Poliovirus (PV) belongs to the Enterovirus genus of the Picornaviridae family. The PV genome, approximately 7.5 kb in length, is a single-stranded, positive-sense RNA enclosed within a capsid protein shell. The P1 is further cleaved by a viral protease to produce the capsid subunit proteins VP0, VP1, and VP3. In this study, we investigate the production, antigenicity, thermostability, immunogenicity, and structures of VLPs derived from PV serotype 2 (PV2) wildtype strain and thermally stabilized mutant (wtVLP and sVLP, respectively).

The structural comparison showed that the wtVLP is highly similar to the PV1 135S-like particles, and the sVLP structure aligns well with the native PV2 model. These data indicate that the PV2 sVLP adopts a native conformation similar to that of the corresponding mature virion, whereas the PV2 wtVLP is in a non-native expanded state. However, the wtVLP appears to be in an expanded state compared to the sVLP, as evidenced by the radius of the wtVLP being 170 Å and that of the sVLP being 163 Å. Structural comparison revealed that the two-fold axis channel, formed by VP2 and VP3, is markedly opened in the wtVLP, whereas it is closed in the sVLP. Noteworthy, a lipid “pocket factor” modeled as sphingosine was observed within the VP1 “pocket” of the sVLP, while the “pocket” in the wtVLP was empty. In comparison to the PV2 wtVLP, the sVLP contains five amino acid alterations, including VP1 T41I, VP1 F134L, VP1 Y159F, VP3 L85F, and VP3 Q178L. According to our structural analysis, VP1 F134L and Y159F are situated in the VP1 pocket, VP3 Q178L is located at the protomer interface and in proximity to the quasi-three-fold, L85F is present on the VP3 β-sheet, and VP1 T41I, which remains unresolved, is at the pentamer interface within the capsid. In the sVLP, the Q178L mutation transforms the residue from a hydrophilic to a hydrophobic amino acid, thereby enhancing the hydrophobic interaction between protomers. In addition, the residues F134L and Y159F enlarge the “pocket” to accommodate a lipidic pocket factor, which is known to stabilize the particle. While VP4 and the N-terminal (residues 1–68) of VP1 are unresolved in both VLPs, the sVLP, unlike the wtVLP, has ordered structures in the C-terminal of VP1, residues 213–231 in the VP1 GH loop, residues 134–149 and 160–173 in the VP2 EF loop, and the VP3 GH loop. Interestingly, the doorloop 232–236 in our PV2 sVLP was found to be in the “down” conformation whereas it adopts the “up” conformation in the PV2 native virion model.

> GLGDLIEGVVEGVTRNALTPLTPANNLPDTQSSGPAHSKEIPALTAVETGATNPLVPSDTVQTRHVIQKRTRSESTVESFFARGACVAIIEVDNDAPTKRASKLFSVWKITYKDTVQLRRKLEFFTYSRFDMELTFVVTSNYTDANNGHALNQVYQIMFIPPGAPIPGKWNDYTWQTSSNPSVFYTYGAPPARISVPYVGIANAYSHFYDGFAKVPLAGQASTEGDSLYGAASLNDFGSLAVRVVNDHNPTKLTSKIRVYMKPKHVRVWCPRPPRAVPYYGPGVDYKDGLAPLPEKGLTTY;> SPNIEACGYSDRVMQLTLGNSTITTQEAANSVVAYGRWPEYIKDSEANPVDQPTEPDVAACRFYTLDTVTWRKESRGWWWKLPDALKDMGLFGQNMFYHYLGRAGYTVHVQCNASKFHQGALGVFAVPEMCLAGDSTTHMFTKYENANPGEKGGEFKGSFTLDTNATNPARNFCPVDYLFGSGVLAGNAFVYPHQIINLRTNNCATLVLPYVNSLSIDSMTKHNNWGIAILPLAPLDFATESSTEIPITLTIAPMCCEFNGLRNITVPRTQ;> GLPVLNTPGSNQYLTADNYQSPCAIPEFDVTPPIDIPGEVRNMMELAEIDTMIPLNLTNQRKNTMDMYRVELNDAAHSDTPILCFSLSPASDPRLAHTMLGEILNYYTHWAGSLKFTFLFCGSMMATGKLLVSYAPPGAEAPKSRKEAMLGTHVIWDIGLQSSCTMVVPWISNTTYRLTINDSFTEGGYISMFYQTRVVVPLSTPRKMDILGFVSACNDFSVRLLRDTTHISQEAMPQ> TEAAAQPHALPADAPDIAPERDLLSKFDGLIAERQKLLDSGVTDPFAIVMEQVKSPTEAVIRGKDTILLGTYNYMGMTFDPDVIAAGKEALEKFGSGTCGSRMLNGTFHDHMEVEQALRDFYGTTGAIVFSTGYMANLGIISTLAGKGEYVILDADSHASIYDGCQQGNAEIVRFRHNSVEDLDKRLGRLPKEPAKLVVLEGV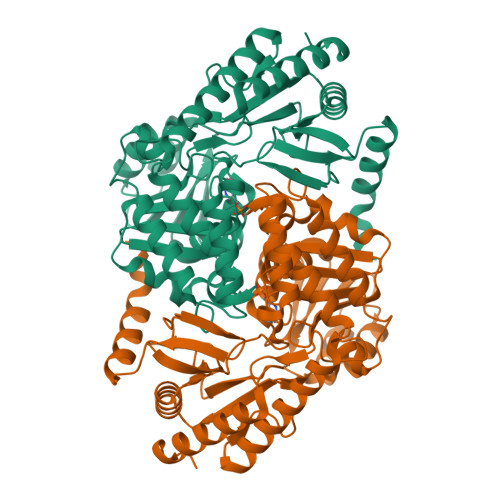YSMLGDIAPLKEMVAVAKKHGAMVLVDEAHSMGFFGPNGRGVYEAQGLEGQIDFVVGTFSKSVGTVGGFVVSNHPKFEAVRLACRPYIFTASLPPSVVATATTSIRKLMTAHEKRERLWSNARALHGGLKAMGFRLGTETCDSAIVAVMLEDQEQAAMMWQALLDGGLYVNMARPPATPAGTFLLRCSICAEHTPAQIQTVLGMFQAAGRAVGVIGLEHHHHHH>MTKNSSLLAEFPTCPRDEKDRPRVFTAASGAWLTDESGFRWIDFDNARGSILLGHGDPVVAEAVARAATGADGTATGWSRRVDAVLERLHALCGGEVVGLFRSGTAAVRAAVLAVREATGRPLLLSAGYHGYDPMWYPSEAPLEPNADGVVDFFFDLGLLRELLRAPERVAAVVVSPDHMHLSPGWYRELRRLCSAAGVVLVADEVKVGLRYAPGLSTAELLAPDVWVVAKGMANGHAVSAVGGSRRLLKPLKEVSFTSFFEPTILAAADAALARVATGEPQRAVREAGDRFLRHARKALDDASLPVEIAGDGTFFQFVPATEELEEALYGAANAEGLLFYAGDNQGVS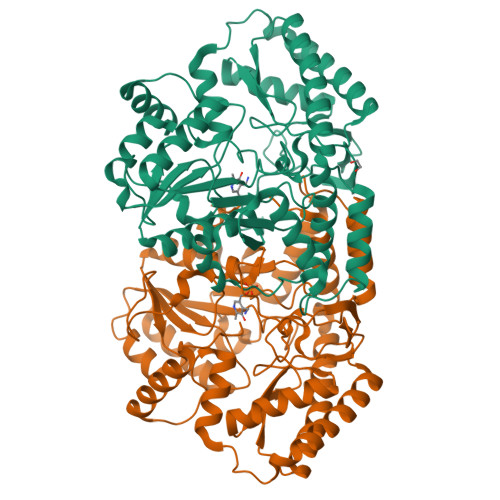AAFDEAVLGEAERRFARVCERLAPYAGGEPVGDAARYRVAWNVMDGLRQAPRDREETTGLLARLLDDLEHHHHHH[4x]>[2x]SMRTAQEVETYRRSKEITVRGHNCPKPVLNFYEANFPANVMDVIARQNFTEPTAIQAQGWPVALSGLDMVGVAQTGSGKTLSYLLPAIVHINHQPFLERGDGPICLVLAPTRELAQQVQQVAAEYCRACRLKSTCIYGGAPKGPQIRDLERGVEICIATPGRLIDFLECGKTNLRRTTYLVLDEADRMLDMGFEPQIRKIVDQIRPDRQTLMWSATWPKEVRQLAEDFLKDYIHINIGALEL

DExD/H-box RNA helicases, from virus and bacteria to eukaryotes, play important roles in processes including ribosome biogenesis, RNA processing and folding, ribonucleoprotein (RNP) remodeling, RNA nuclear export, the regulation of RNA translation and transcription, and nonsense-mediated RNA decay. DExD/H-box proteins often contain accessory regulatory domains and localization modules, but their cores consist of two RecA-like domains joined by a short flexible linker. The N-terminal domain is commonly referred to as conserved domain-1, or DEAD-domain, and the C-terminal domain as conserved domain-2, or helicase domain. Both domains contribute to the binding site for RNA substrates and both contribute to ATP hydrolysis. We used X-ray crystallography to determine the structures of the DEAD-domains of DDX2A, DDX2B, DDX5, DDX10, DDX18, DDX20, DDX47, DDX52, and DDX53, as well as the helicase domains of DDX25 and DDX41.

DDX5 is a co-regulator of different transcription factors including ERα, p53, MyoD and Runx2, but ATPase/helicase activity is not required for transcriptional co-regulation. DDX5 also participates in pre-RNA processing, alternative splicing, microRNA and ribosomal RNA processing. In the crystal complexes with either ADP or AMP the loop closes up, resulting in a shift in Cα-atom positions by up to 3.5 Å between the ATP- and the AMP-states, or by up to 2.5 Å between the ADP- and the AMP-state. Thus the conformation of the P-loop is determined by the nucleotide phosphates, and longer phosphate tails result in a more open loop. Inspection of the RNA complexes of DDX19, vasa, and eIF4AIII shows that the conserved motif that makes the most extensive contacts with the RNA-backbone phosphates is motif Ib. In two of our DEAD-domain crystal structures, anions from the crystallization buffers are bound to motif Ib (a sulfate in DDX5, and a phosphate in DDX47) highlighting the ability of this motif to bind polyanions.CIS-2,6-DIMETHYLMORPHOLINOOCTYLCARBAMYLESEROLINE 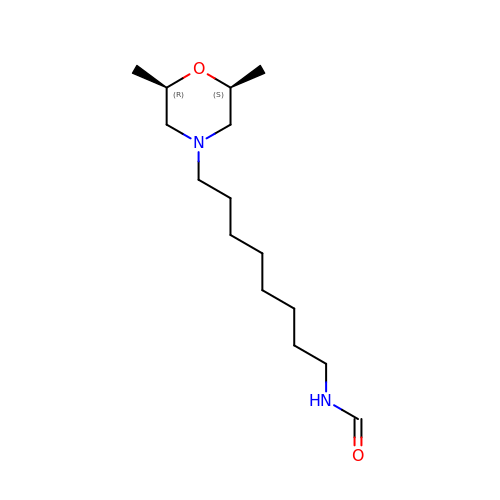| C15 H30 N2 O2 | UXVBAZRPAJEAHR-GASCZTMLSA-N> GSHMWDTANNPL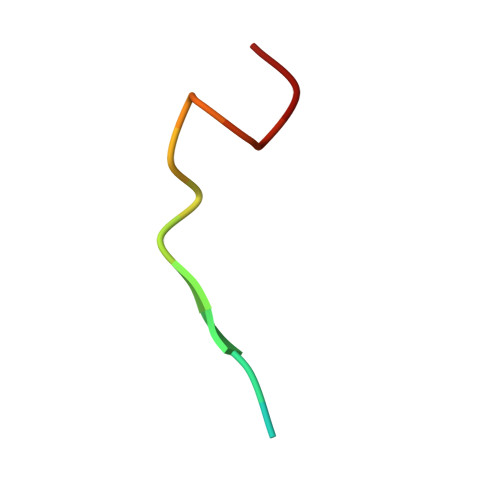YKEA(1S,2S,3R,4S,6R)-4,6-diamino-3-{[(2S,3R)-3-amino-6-(hydroxymethyl)-3,4-dihydro-2H-pyran-2-yl]oxy}-2-hydroxycyclohexyl 3-deoxy-4-C-methyl-3-(methylamino)-beta-L-arabinopyranoside | C19 H36 N4 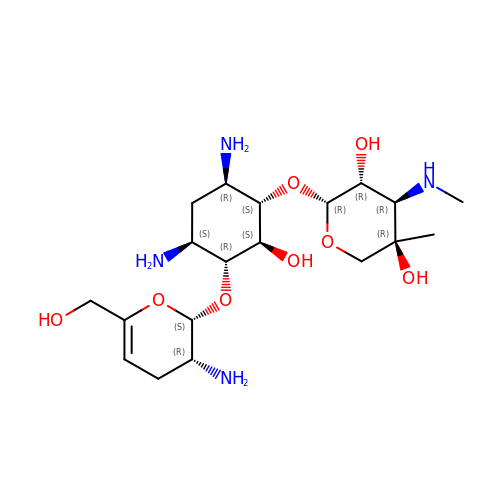O8 | IZDCJSIPHXBXBL-YFMIWBNJSA-N Slx1 harbors an N-terminal catalytic GIY-YIG endonuclease domain followed by a C-terminal zinc finger motif. Individual Slx1 has very weak nuclease activity, while association with Slx4 could dramatically enhance its enzymatic activity. Slx1 C-terminal zinc finger and Slx4 C-terminal helix-turn-helix domain are well conserved throughout evolution, and have been mapped out to be the minimal fragment of each protein required for the complex formation. Here, we report the crystal structure of the Schizosaccharomyces pombe Slx1 C-terminal RING finger domain in complex with Slx4 C-terminal four-helix bundle domain, which provides structural insights into the Slx1-Slx4 complex formation.

To provide structural insights into the protein component and complex architectures, we determined the crystal structure of Slx1RING-Slx4CCD complex to 2.0 Å resolution. Each asymmetric unit of the crystal is composed of two nearly identical Slx1-Slx4 heterodimers, with residues Val178–Thr246 of Slx1 and Ile352-Ser417 of Slx4 well fitted in the final structure model. Slx1RING adopts a compact α/β structural fold, consisting of two two-stranded antiparallel β1-β2 and β3-β4 sheets and two α helices. Slx1RING possesses a RING finger structural topology, which includes the pattern of chelating two zinc atoms and has a characteristic helix α1. Homology search with Dali server indicated that Slx1 zinc finger shares the most similar fold with a consistent series of RING finger proteins (e.g. FANCL, RNF4, and RING1b), while Slx1 RING finger contains an unusual long loop following helix α1 which is directly involved in the interaction with Slx4CCD. Slx4CCD is folded as a helix-turn-helix domain containing a four-helix bundle (α1–α4), with residues from helices α1, α2, and α4 constituting the Slx1RING binding interface. Slx1RING-Slx4CCD heterodimer buries a total accessible surface area of ~1470 Å2. Both hydrophobic interactions and hydrogen bonding contribute to the complex formation. The long loop (Thr216-Ile224) with negative electrostatic potential protrudes and binds to Slx4CCD helix α1 area with strong positive electrostatic potential, which contributes to the formation of complex interface. Slx1 C-terminal domain was originally classified into a PHD finger based on the primary sequence information, but the structural information we provided here indicated it possesses structural characteristics of C4HC3-type RING fingers.

>MEPVKCNLCYECIESDELRANCPFTDCNSINHLTCLASSFLTEECQVLPIEGMCTKCKRVLRWREFLSTVFTT[2x];>[2x]GSMIVTQTHRAISQVVKQAKDNSVWIKILTYSAIDVEEFQLWLKRKNLNVSLDLIKSWCDKYGVLMKGSWH> MDVAGLTD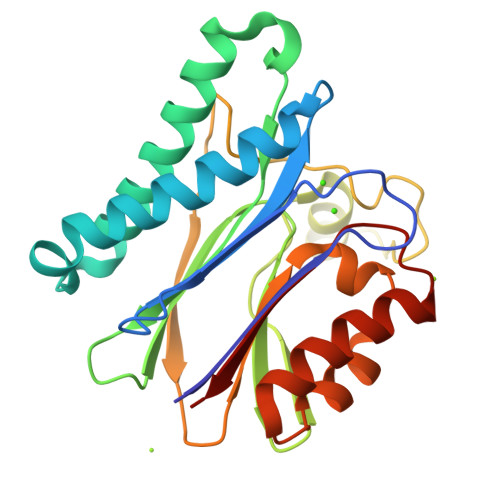CGLIRKSNQDAFYIDEKHQRFFIVADGMGGHAGGEEASRLAVDHIRQYLETHLEDLQHDPVTLLRQAFLAANHAIVEQQRQNSARADMGTTAVVILLDEKGDRAWCAHVGASRIYRWRKDQLQQITSDHTWIAQAVQLGSLTIEQARQHPWRHVLSQCLGREDLSQIDIQPIDLEPGDRLLLCSDGLTEELTDDVISIYLSEPNVQKAAAALVDAAKTHGGRDNVTVVVISV>GHMSTFLPAPLQCGRFELTFERPLVMGILNATPDSFSDGGRFLARDDALRRAERMIAEGADLLDIGGESTRPGAPPVPLDEELARVIPLVEALRPLNVPLSIDTYKPAVMRAALAAGADLINDIWGFRQPGAIDAVRDGNSGLCAMHMLGEPQTMQVGEPDYGDVVTDVRDFLAARAQALRDAGVAAERICVDPGFGFGKAVVDDNYALLAALPDTAPARPDGRAYPILAGMSRKSMLGAVIGGKPPLERVAASVAAALCAVERGAAIVRVHDVAATVDALSVWNAVRAAARQR[2x]

Dihydropteroate synthase (DHPS, EC: 2.5.1.15) catalyses the reaction of 6-hydroxymethyl-7,8-dihydropterin-pyrophosphate with p-aminobenzoic acid (p-ABA) to yield 7,8-dihydropteroate and pyrophosphate. In so doing the enzyme supports the biosynthesis of folate, a key metabolite required to support the synthesis of DNA, and proteins. BcDHPS displays a triosephosphate isomerase (TIM)-barrel fold, consisting of eight parallel β-strands surrounded by eight α-helices. The DHPS active site is formed entirely within a single subunit.

The structure of BcDHPS complexed with 7,8-dihydropteroate was refined to 1.95 Å resolution. The crystals for the complex structure display space group P212121 and there are two molecules, labeled A and B, in the asymmetric unit. Here, the product of the enzyme reaction, 7,8-dihydropteroate is ordered, placed with the pterin directed down into the barrel with the p-ABA moiety pointing out towards the surface of the protein. The ligand possesses nine functional groups of which eight participate in direct hydrogen bonds with DHPS. Four hydrogen bond donors, N2, N3, N8 and N14 interact with functional groups on Asn120, Asp191, Asp101 and Thr68 respectively. On the other side of the pterin, O4 and N5 accept hydrogen bonds donated from Lys233 NZ. A carboxylate oxygen, on the p-ABA moiety, accepts hydrogen bonds donated from the main chain amide and side chain hydroxyl groups of Ser234. The pterin is sandwiched between a cluster of hydrophobic residues (Ile122, Met144 and Phe196) on one side and the guanidinium group of Arg268 on the other (data not shown). Modeling of loop 2, linking β2 to α2 was possible only in the case of the product complex. We were fortunate that the product complex of BcDHPS allowed us to model loop 2 and the complete structure we obtained provides an improved template suited for in silico screening.> SPLVQLAGIRKCFDGKEVIPQLDLTINNGEFLTLLGPSGCGKTTVLRLIAGLETVDSGRIMLDNEDITHVPAENRYVNTVFQSYALFPHMTVFENVAFGLRMQKTPAAEITPRVMEALRMVQLETFAQRKPHQLSGGQQQRVAIARAVVNKPRLLLLDQSLSALDYKLRKQMQNELKALQRKLGITFVFVTHDQEEALTMSDRIVVMRDGRIEQDGTPREIYEEPKNLFVAGFIGEINMFNATVIERLDEQRVRANVEGRECNIYVNFAVEPGQKLHVLLRPEDLRVEEINDDNHAEGLIGYVRERNYKGMTLESVVELENGKMVMVSEFFNEDDPDFDHSLDQKMAINWVESWEVVLAD;> FQNVVIVTIVGWLVLFVFLPNLMIIGTSFLTRDDASFVKMVFTLDNYTRLLDPLYFEVLLHSLNMALIATLACLVLGYPFAWFLAKLPHKVRPLLLFLLIVPFWTNSLIRIYGLKIFLSTKGYLNEFLLWLGVIDTPIRIMFTPSAVIIGLVYILLPFMVMPLYSSIEKLDKPLLEAARDLGASKLQTFIRIIIPLTMPGIIAGCLLVMLPAMGLFYVSDLMGGAKNLLIGNVIKVQFLNIRDWPFGAATSITLTIVMGLMLLVYWRASRLLN;> LLRGGFMTAIYAYLYIPIIILIVNSFNSSRFGINWQGFTTKWYSLLMNNDSLLQAAQHSLTMAVFSATFATLIGSLTAVALYRYRFRGKPFVSGMLFVVMMSPDIVMAISLLVLFMLLGIQLGFWSLLFSHITFCLPFVVVTVYSRLKGFDVRMLEAAKDLGASEFTILRKIILPLAMPAVAAGWVLSFTLSMDDVVVSSFVTGPSYEILPLKIYSMVKVGVSPEVNALATILLVLSLVMVIASQLIAR;> PLVQLAGIRKCFDGKEVIPQLDLTINNGEFLTLLGPSGCGKTTVLRLIAGLETVDSGRIMLDNEDITHVPAENRYVNTVFQSYALFPHMTVFENVAFGLRMQKTPAAEITPRVMEALRMVQLETFAQRKPHQLSGGQQQRVAIARAVVNKPRLLLLDQSLSALDYKLRKQMQNELKALQRKLGITFVFVTHDQEEALTMSDRIVVMRDGRIEQDGTPREIYEEPKNLFVAGFIGEINMFNATVIERLDEQRVRANVEGRECNIYVNFAVEPGQKLHVLLRPEDLRVEEINDDNHAEGLIGYVRERNYKGMTLESVVELENGKMVMVSEFFNEDDPDFDHSLDQKMAINWVESWEVVLA

The PotD-PotABC protein complex in Escherichia coli, belonging to the adenosine triphosphate–binding cassette transporter family, is a spermidine-preferential uptake system. In general, ATP binding, hydrolysis, and phosphate release trigger conformational changes in the transporter, leading to the uptake of extracellular polyamines. Here, we report structural details of the polyamine uptake system PotD-PotABC in various states.

We also successfully modeled the structure of the PotABC complex with the bound ligand Spd. In the Spd-bound complex, one Spd molecule is enclosed within the membrane cavity, formed mainly by transmembrane helices 3 to 5 (TM3 to TM5) of both PotB and PotC. The residues S113 and Y223 in PotB, along with D198 in PotC, establish interactions with Spd amine at one end, while residues M104, S106, and D108 in PotC interact with the other end. D108 also interacts with the middle amine group. In addition, residues I160, F164, and L213 in PotB engage in hydrophobic interactions with the carbon atoms of Spd. Together, PotB (F164 and L213) and PotC (F142 and L191) block Spd exit into the cytosol. Despite adding ATP to the sample before vitrification, no corresponding density indicative of ATP was observed in PotA. In particular, the residue Y223 in PotB faces inward to form a hydrogen-bonding interaction with the Spd terminal amide group. As the translocation pathway opens further on the cytoplasmic side, the residues (PotB F164 and L213; and PotC F142 and L191) move apart, allowing Spd to be released to the cytosol.>FPDNAVPYPWSNAQLSWQRTAFHFQPERSWMSDPDGPIFYKGWYHFFYQYNPDNPVWGNNTWGHTVSRDLIHWLYLPLALAADQWYDMQGVFSGSATCLPDGRIMMLYTGVTKEMVEMLSLAYPADLSDPLLVEWVKYPGNPILSAPPGVSPTEFRDASTGWYVSNGTWRIAIGAKYNTTGIAMVYETKDFKSFKLLEELLHAVPDTGLWECVDLYPVSTTGEKGLETSVNGPKVKHVLKASIDEQQRDYYAIGTYDLGTNKWTPDNPEEDVGIGLRYDWGKYYASKTFYDPKKQRRVVWAWTKELDSEVADREKGWANVQTIPRTVLLDQKTGTNVLLWPVEEVES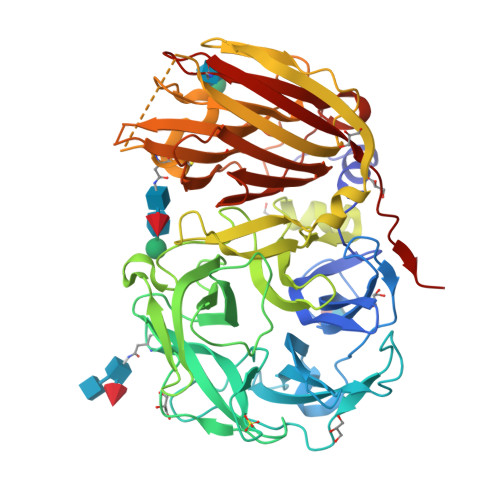LRLSSKEFSKVKAGAGSVVPLDVGTATQLDIIAEFEIDKEALEGTIEADMGYNCTTSGGAAERGVLGPFGLLVSATENLSEQTPVYFYIAKGTDGNFKTFFCLDESRSSKASDVSKQVKGFTVPVLDGEKFTMRLLVDHSIVESFAQGGRSCITSRVYPTEAIYGAAKLFLFNNATGASITASLKIWEMNSAFIQPFHR[2x]N-[(1S)-2-amino-1-phenylethyl]-5-(1H-pyrrolo[2,3-b]pyridin-4-yl)thiophene-2-carboxamide | C20 H18 N4 O S | 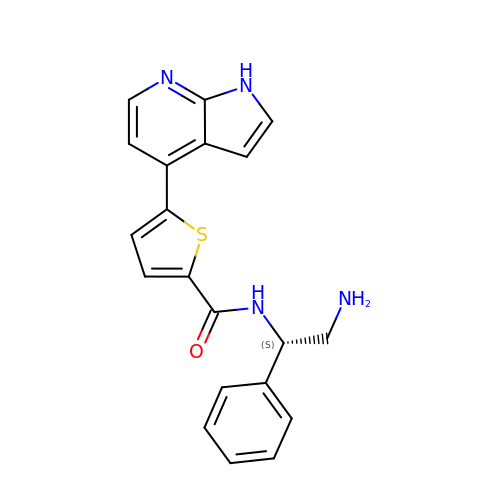TWYNGDRSMHRPSY-MRXNPFEDSA-N> RSMQQNDYNQNRGEHIDWQDDDVSKIKQQEDFDFQR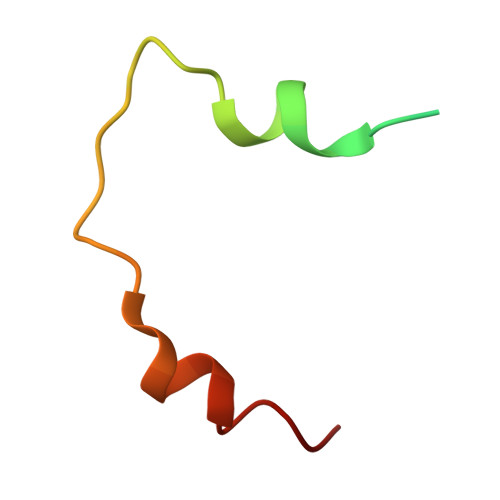NLGMFNK>[2x]DPPATVYRYDSRPPEDVFQNGFTAWGNNDNVLEHLTGRSCQVGSSNSAFVSTSSSRRYTEVYLEHRMQEAVEAERAGRGTGHFIGYIYEVRADNNFYGAASSYFEYVDTYGDNAGRILAGALATYQSEYLAHRRIPPENIRRVTRVYH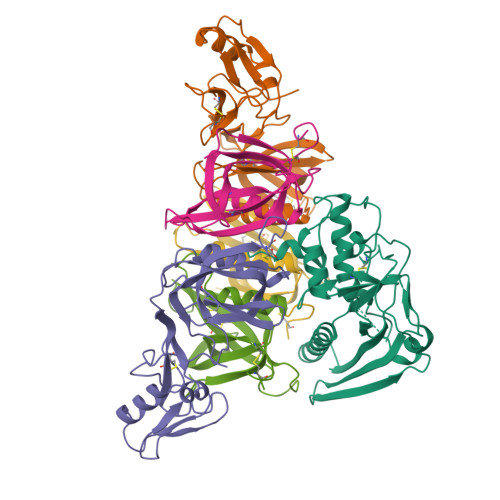NGITGETTTTEYSNARYVSQQTRANPNPYTSRRSVASIVGTLVRMAPVVGACMARQAESSEAMAAWSERAGEAMVLVYYESIAYSF;>GIVIPPQEQITQHGSPYGRCANKTRALTVAELRGSGDLQEYLRHVTRGWSIFALYDGTYLGGEYGGVIKDGTPGGAFDLKTTFCIMTTRNTGQPATDHYYSNVTATRLLSSTNSRLCAVFVRSGQPVIGACTSPYDGKYWSMYSRLRKMLYLIYVAGISVRVHVSKEEQYYDYEDATFETYALTGISICNPGSSLC[2x];>GIVIPPKALFTQQGGAYGRCPNGTRALTVAELRGNAELQTYLRQITPGWSIYGLYDGTYLGQAYGGIIKDAPPGAGFIYRETFCITTIYKTGQPAADHYYSKVTATRLLASTNSRLCAVFVRDGQSVIGACASPYEGRYRDMYDALRRLLYMIYMSGLAVRVHVSKEEQYYDYEDATFQTYALTGISLCNPAASIC[2x];>[4x]DVPYVLVKTNMVVTSVAMKPYEVTPTRMLVCGIAAKLGAAASSPDAHVPFCFGKDLKRPGSSPMEVMLRAVFMQQRPLRMFLGPKQLTFEGKPALELIRMVECSGKQDCP;>[2x]LPTHLYKNFTVQELALKLKGKNQEFCLTAFMSGRSLVRACLSDAGHEHDTWFDTMLGFAISAYALKSRIALTVEDSPYPGTPGDLLELQICPLNGYCE>MSEPSEKKQKVATSSLEQLKKAGTHVVADSGDFEAISKYEPQDSTTNPSLILAASKLEKYARFIDAAVEYGRKHGKTDHEKIENAMDKILVEFGTQILKVVPGRVSTEVDARLSFDKKATVKKALHIIKLYKDAGVPKERVLIKIASTWEGIQAARELEVKHGIHCNMTLLFSFTQAVACAEANVTLISPFVGRI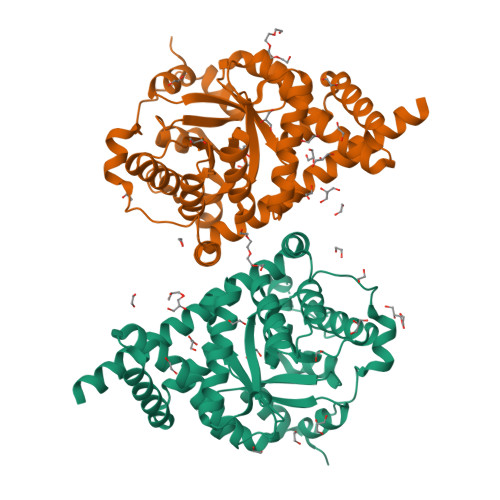MDFYKALSGKDYTAETDPGVLSVKKIYSYYKRHGYATEVMAASFRNLDELKALAGIDNMTLPLNLLEQLYESTDPIENKLNSESAKEEGVEKVSFINDEPHFRYVLNEDQMATEKLSDGIRKFSADIEALYKLVEEKMLEHHHH[2x]Transporters of the Nramp (Natural resistance-associated macrophage protein) family import divalent transition metal ions into cells of most organisms. In addition to the physiological substrates Fe2+ and Mn2+, Nramps can also transport toxic metals like Cd2+ and Hg2+ but exclude the abundant alkaline earth metals like Mg2+ and Ca2+. Recent bacterial Nramp structures reveal a LeuT fold, three stable conformations (outward-open, occluded, and inward-open), and identify the metal-binding site residues, including conserved aspartate, asparagine, and methionine residues. We present high-resolution structures of DraNramp in three conformations in both Mn2+-bound and metal-free states, providing the first molecular map of the entire Mn2+ transport cycle.

To compare the metal-bound states to analogous metal-free states of the transport cycle, we determined two metal-free occluded structures of wildtype DraNramp at a higher resolution than the previously reported G45R structure, which we refer to as WT (2.38 Å) and WTsoak (2.36 Å). WT and WTsoak are nearly identical, confirming that the soaking process does not influence the conformational state. In the occluded structure of metal-free WT DraNramp a density we have assigned as water replaces Mn2+. In contrast, metal-free WT has a more ordered orthosteric site, suggesting a stable occluded intermediate in the switch from inward- to outward-open. Interestingly, both metal-free and Mn2+-bound WT DraNramp crystallized in the occluded conformation, whereas the open conformations were achieved through conformation-locking or mutations of functionally important residues. Overall, our DraNramp structures suggest that the occluded state is most stable (at least in the absence of a membrane potential).

> MHHHHHHHHAGPRGVRRILPFLGPAVIASIAYMDPGNFATNIEGGARYGYSLLWVILAANLMAMVIQNLSANLGIASGRNLPELIRERWPRPLVWFYWIQAELVAMATDLAEFLGAALAIQLLTGLPMFWGAVVTGVVTFWLLNLQKRGTRPLELAVGAFVLMIGVAYLVQVVLARPDLAAVGAGFVPRLQGPGSAYLAVGIIGATVMPHVIYLHSALTQGRIQTDTTEEKRRLVRLNRVDVIAAMGLAGLINMSMLAVAAATFHGKNVENAGDLTTAYQTLTPLLGPAASVLFAVALLASGLSSSAVGTMAGDVIMQGFMGFHIPLWLRRLITMLPAFIVILLGMDPSSVLILSQVILCFGVPFALVPLLLFTARRDVMGALVTRRSFTVIGWVIAVIIIALNGYLLWELLGG> GPMARSLIKTDWSGSEYTILGAN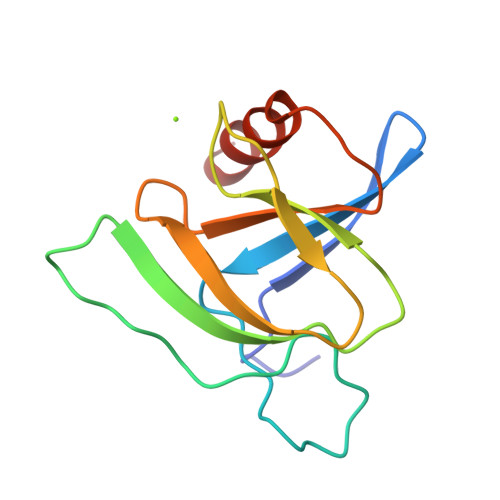HYEEPNTGAAAQFPGTMAEDDGRSPYIVRKLRNSSGKRFYVFTDHPQQPIIWNPHEEIEIQFSRKYLIAVLTEFEADSKVFTHFARRQHRS> GAMDGLTGATKIKLESSAKAIVDEIDAIKKKAASMGVNFDAFKDKKTGSGVSE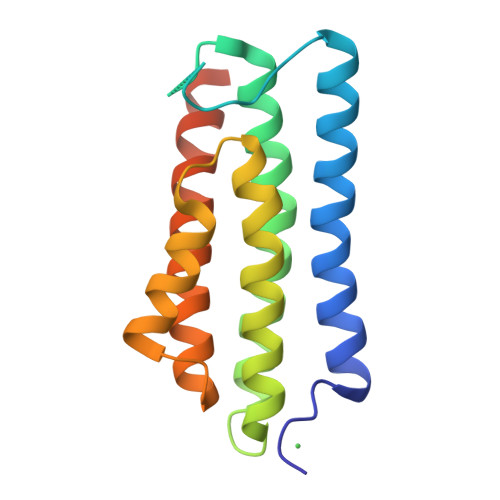NPFILEAKVRATTVAEKFVIAIEEEATKLKETGSSGEFSAMYDLMFEVSKPLQELGIQEMTKTVSMAAEENPPTTAQGVLEIAKKMREKLQRVHKKNQDTLKKKNTEDSTAKS>MPFEFENLGMGIILIKPKVFPDKRGFFLEVFKSEDFTKMRIPNVIQTNMSFSRKGVVRGLHYQRTPKEQ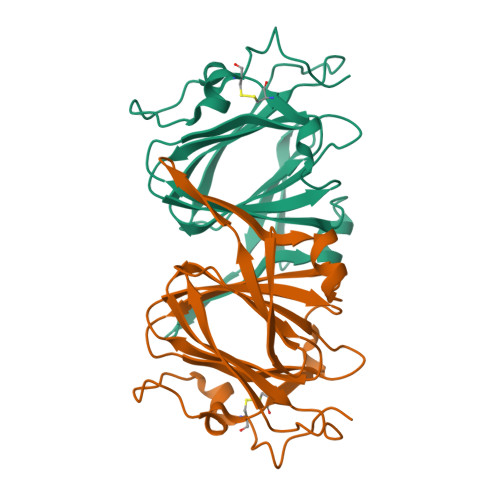GKIIFVPKGRILDVAVDVRKSSPTFGKYVKAELNEENHYMLWIPPGFAHGFQALEDSIVIYFITHNEYSPPHERCISYSYIDWPIKEVIISDKDLQCPSLEKAEVFD[12x]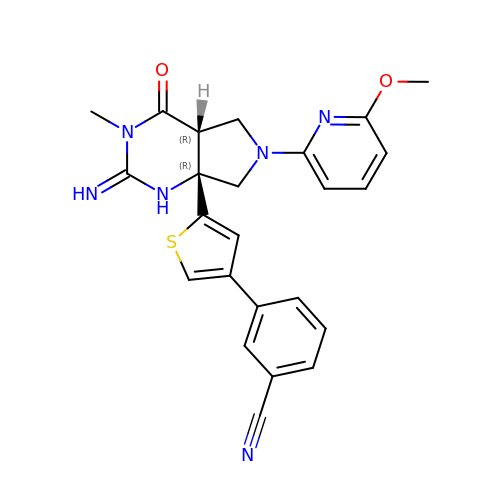3-{5-[(2E,4aR,7aR)-2-imino-6-(6-methoxypyridin-2-yl)-3-methyl-4-oxooctahydro-7aH-pyrrolo[3,4-d]pyrimidin-7a-yl]thiophen-3-yl}benzonitrile | C24 H22 N6 O2 S | DHDYCYIAHXOSEU-UUOWRZLLSA-N>[6x]MSELFSE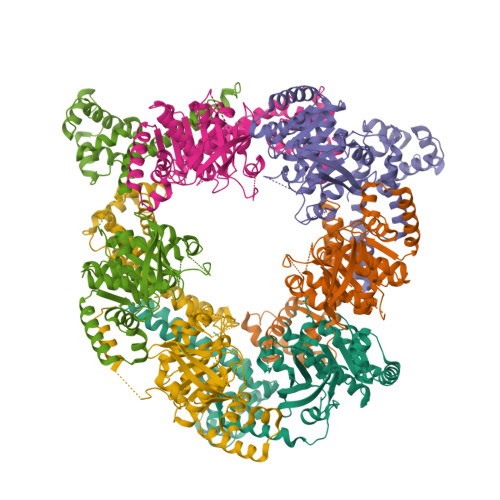RIPPQSIEAEQAVLGAVFLDPAALVPASEILIPEDFYRAAHQKIFHAMLRVADRGEPVDLVTVTAELAASEQLEEIGGVSYLSELADAVPTAANVEYYARIVEEKSVLRRLIRTATSIAQDGYTREDEIDVLLDEADRKIMEVSQRKHSGAFKNIKDILVQTYDNIEMLHNRDGEITGIPTGFTELDRMTSGFQRSDLIIVAARPSVGKTAFALNIAQNVATKTNENVAIFSLEMSAQQLVMRMLCAEGNINAQNLRTGKLTPEDWGKLTMAMGSLSNAGIYIDDTPSIRVSDIRAKCRRLKQESGLGMIVIDYLQLIQGSGRSKENRQQEVSEISRSLKALARELEVPVIALSQLSRSVEQRQDKRPMMSDIRESGSIEQDADIVAFLYRDDYYNKDSENKNIIEIIIAKQRNGPVGTVQLAFIKEYNKFVNLERRFDEAQIPPGA> MANRATSAFLDNPHPVGVNYVDEGSRQFVAVAELLASKLIDSSRESDESNSDVPFVQAYSKFADDNPRHLRVKTGGKMANALTNVIRSYYSINAPAIVPQVEIDRLASKATVSGDMYNSYAIFNSVPIVEVLSPARTTVSIVGSDRADVTMLNTGAGAANITFNFGQIAETVILKGSVPFQLARLNQPMPAARFTYKLRPLDGPFIVVLPVGNPLVISATAATRIQVPLAFNKALVESGFQTAMNDGLFDIQNVNYYSSFDEFIISQYHAQDGIN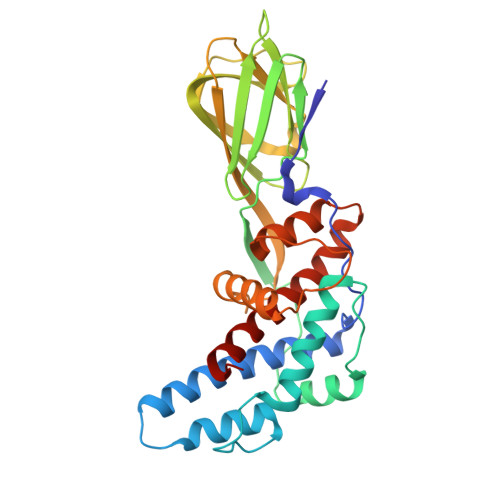RVSTCVILGLALQAYDQMRRALPVRR> MREPEELMPDSGAVFTFGKSKFAENNPGKFWFKNDVPVHLSCGDEHSAVVTGNNKLYMFGSNNWGQLGLGSKSAISKPTCVKALKPEKVKLAACGRNHTLVSTEGGNVYATGGNNEGQLGLGDTEERNTFHVISFFTSEHKIKQLSAGSNTSAALTEDGRLFMWGDNSEGQIGLKNVSNVCVPQQVTIGKPVSWVSCGYYHSAFVTTDGELYVFGEPENGKLGLPNQLLGNHRTPQLVSEIPEKVIQVACGGEHTVVLTENAVYTFGLGQFGQLGLGTFLFETSEPKVIENIRDQTISYISCGENHTALITDIGLMYTFGDGRHGKLGLGLENFTNHFIPTLCSNFLRFIVKLVACGGCHMVVFAAPHRGVAKEIEFDEINDTCLSVATFLPWSHPQ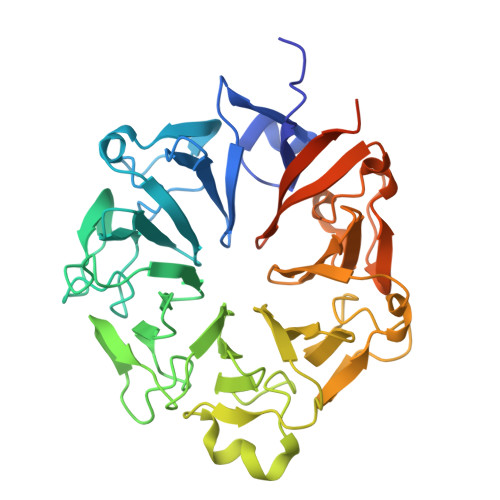FEK>GAEIYNKDGNKVDLYGKAVGLHYFSKGNGENSYGGNGDMTYARLGFKGETQINSDLTGYGQWEYNFQGNNSEGADAQTGNKTRLAFAGLKYADVGSFDYGRNYGVV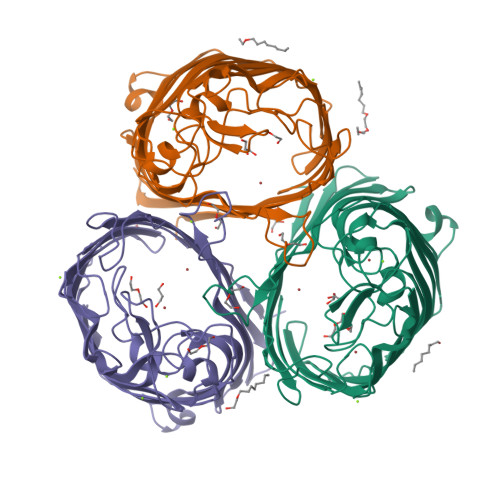YDALGYTDMLPEFGGDTAYSDDFFVGRVGGVATYRNSNFFGLVDGLNFAVQYLGKNERDTARRSNGDGVGGSISYEYEGFGIVGAYGAADRTNLQEAQPLGNGKKAEQWATGLKYDANNIYLAANYGETRNATPITNKFTNTSGFANKTQDVLLVAQYQFDFGLRPSIAYTKSKAKDVEGIGDVDLVNYFEVGATYYFNKNMSTYVDYIINQIDSDNKLGVGSDDTVAVGIVYQF[3x]>[4x]MATANGAVENGQPDRKPPALPRPIRNLEVKFTKIFINNEWHESKSGKKFATCNPSTREQICEVEEGDKPDVDKAVEAAQVAFQRGSPWRRLDALSRGRLLHQLADLVERDRATLAALETMDTGKPFLHAFFIDLEGCIRTLRYFAGWADKIQGKTIPTDDNVVCFTRHEPIGVCGAITPWNFPLLMLVWKLAPALCCGNTMVLKPAEQTPLTALYLGSLIKEAGFPPGVVNIVPGFGPTVGAAISSHPQINKIAFTGSTEVGKLVKEAASRSNLKRVTLELGGKNPCIVCADADLDLAVECAHQGVFFNQGQCCTAASRVFVEEQVYSEFVRRSVEYAKKRPVGDPFDVKTEQGPQIDQKQFDKILELIESGKKEGAKLECGGSAMEDKGLFIKPTVFSEVTDNMRIAKEEIFGPVQPILKFKSIEEVIKRANSTDYGLTAAVFTKNLDKALKLASALESGTVWINCYNALYAQAPFGGFKMSGNGRELGEYALAEYTEVKTVTIKLGDKNP

The ALDH1A subfamily, comprised of isoforms ALDH1A1, ALDH1A2, and ALDH1A3, regulate RA signaling important for embryogenesis and development. Following the first step of oxidation of Vitamin A (retinol) to retinaldehyde by members of the short-chain dehydrogenase/reductase superfamily of proteins, ALDH1A enzymes irreversibly convert retinaldehyde to RA—reviewed in19. Of the many ALDH isoforms, we and others have implicated the elevated expression of ALDH1A3 in mesenchymal glioma stem cells (MES GSCs) as a target for the development of novel therapeutics. The lead compound, MCI-INI-3, is a selective competitive inhibitor of human ALDH1A3 and shows poor inhibitory effect on the structurally related isoform ALDH1A1.

The three-dimensional structure of human ALDH1A3 in a complex with MCI-INI-3 was determined at a resolution of 2.8 Å. The final model contains four identical protein chains per asymmetric unit, arranged in a tetramer, a total of 257 solvent molecules and 4 inhibitor molecules. The molecule (MCI-INI-3) establishes multiple interactions with protein residues. In particular, the ester group of MCI-INI-3 pointed towards the catalytic cysteine at a distance of about 5 Å and its benzodioxole moiety established several contacts with the protein environment, including an H-bond with W189 and Van der Waals contacts with T140 and R139. The phenyl group of MCI-INI-3, which makes a π-π stacking interaction of variable quality with F308, sits close to the protein surface and appears to be rather flexible, being poorly visible in the omit electron density map. With respect to the specific selectivity that MCI-INI-3 shows for ALDH1A3, our structural data revealed that its pyrazolopyrimidine ring contacts N469 (N12-NH2 distance of about 4 Å) and its ester group interacts with T315 (O4-OH distance of about 4 Å), the two amino acids that distinguish the 1A3 isozyme active site. Such stabilizing interactions would simply be impossible in ALDH1A1 where the two structurally equivalent positions are occupied by I304 and G458, residues that cannot establish electrostatic interactions with the hydrophilic portions of the inhibitor. At this point, a complete determination of the Michaelis-Menten kinetics was performed that revealed MCI-INI-3 to be a competitive inhibitor for the aldehyde substrate, with Ki values of 0.55 ± 0.11 μM for ALDH1A3 and 78.2 μM ± 14.4 μM for ALDH1A1.Similar to β-CoV nsp1, α-CoV nsp1 has been identified as an important virulence factor that acts by inhibiting the host protein synthesis function. Here, we are the first to report a 1.8-Å full-length crystal structure for FIPV nsp1 and a 2.1-Å full-length crystal structure of SADS-CoV nsp1. The crystal structures of SADS-CoV nsp1 and FIPV nsp1 reveal that their monomers contain six antiparallel β-strands and two α-helices. The overall structure of α-CoVs nsp1 shared the same fold, with a characteristic six-stranded β-barrel formed by β1 relative to β6, β2 relative to β5, and β3 relative to β4.

FIPV is responsible for the deadly systemic immune-mediated granulomatous disease, which has a mortality rate of nearly 100% in cats. Within the genus α-CoV, feline infectious peritonitis virus (FIPV) is in the α-CoV 1A species, which also contains a few other closely related viruses, such as transmissible gastroenteritis virus (TGEV), porcine respiratory coronavirus (PRCV), and canine coronavirus (CCV). The SADS-CoV nsp1 and FIPV nsp1 structures were refined to 2.1- and 1.8-Å resolutions, respectively. Their space groups are P212121 and C121, respectively. Each asymmetric unit of SADS-CoV nsp1 and the FIPV nap1 structures contained two and four subunits, respectively. With the exception of the regions encompassing amino acids 105 to 110 of SADS-CoV nsp1 and 106 to 110 of FIPV nsp1, all the residues of both nsp1 proteins can be built using the final models. Therefore, we could judge the characteristics of the same subtype and different subtypes of α-CoV by structural comparison. This comparison showed that the overall structure of FIPV nsp1 is conserved relative to that of TGEV nsp1 (with an RMSD of 0.53 Å), but it has several differences compared with PEDV nsp1 (with an RMSD of 1.87 Å). The overall structure of FIPV nsp1 and TGEV nsp1 is highly conserved, which shows that the differential amino acids (Asn2, Cys35, Asp71, Ser91, and Phe102) in TGEV nsp1 and FIPV nsp1 will not affect the stability of their overall structure. From the surface electrostatics, the structure of FIPV nsp1 was more similar to that of TGEV nsp1 and the structure of SADS-CoV nsp1 was more similar to that of PEDV nsp1. Compared with other α-CoV nsp1s, the ability of FIPV nsp1 to inhibit IFN-β and ISRE reporter genes was greatly decreased.

>MHHHHHHMSSKQFKILVNEDYQVNVPSLPFRDVLQDIKYCYRNGFDGYVFVPEYRRDLVDCNRKDHYVIGVLGNGISDLKPVLLTEPSVMLQGFIVRADCNGVLEDFDLKIARTGNG[4x]>[3x]GSDLTYAYLVGL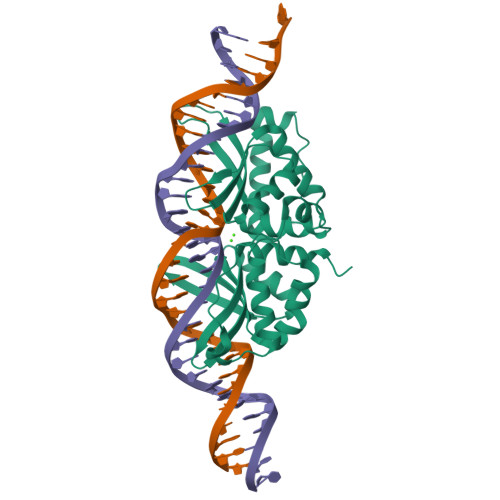YEGDGYFSITKKGKYLTYELGIELSIKDVQLIYKIKKILGIGIVSFRKRNEIEMVALRIRDKNHLKSKILPIFEKYPMFSNKQYDYLRFRNALLSGIIYLEDLPDYTRSDEPLNSIESIINTSYFSAWLVGFIEAEGCFSVYKLNKDDDYLIASFDIAQRDGDILISAIRKYLSFTTKVYLDKTNCSKLKVTSVRSVENIIKFLQNAPVKLLGNKKLQYKLWLKQLRKISRYSEKIKIPSNY> MDHSITASYYDTTQQLSLLKHVLSEDKRPIAFIIAAGCPVSIRHNDAPLIPDVAGLTRKISDSFGGNPDSLLMKIIQNLKTTIPNPTIEDILSY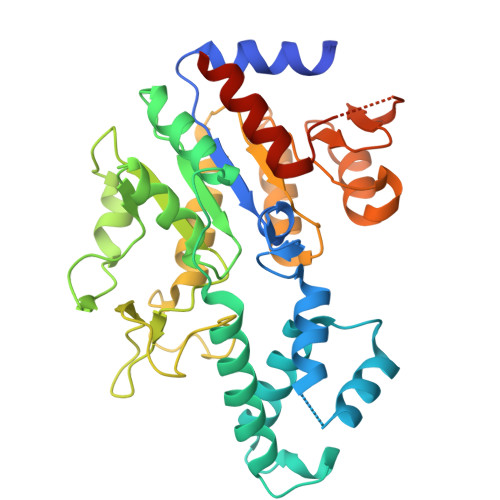IRLLQQIPMSGKIHDVENSVINALEESICELIEEEVNVDLPGNATPYHKIAAWINSINREHQVEIFTTNYDLLMEQALEELNVPYFDGFVGSKRAFFDIRTIEENKLPSRWSKLWKLHGSINWQLDKQTQTIWRGTPSKGCSLIHPSHLKYDQSRKMPYLVMMDQLKLFLNQPSAILITCGYSYKDQHINEVLSQGLQTNPNALIYGLQYDVLENYQEAKDMALKRSNLILLAKDRAIIGKKEGEWKPDPQSSQDNDPLLFFKLGDFQHLASFLEEISQYDWSKQND> SRKKMGLLVMAYGTPYKEEDIERYYTHIRRGRKPEPEMLQDLKDRYEAIGGISPLAQITEQQAHNLEQHLNEIQDEITFKAYIGLKHIEPFIEDAVAEMHKDGITEAVSIVLAPHFSTFSVQSYNKRAKEEAEKLGGLTITSVESWYDEPKFVTYWV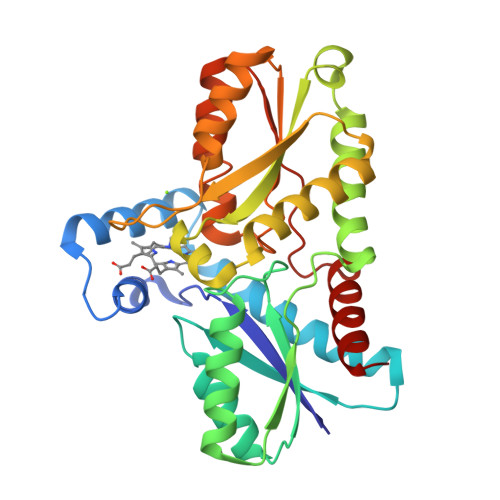DRVKETYASMPEDERENAMLIVSAASLPEKIKEFGDPYPDQLHESAKLIAEGAGVSEYAVGWQSEGNTPDPWLGPDVQDLTRDLFEQKGYQAFVYVPVGFVADHLEVLYDNDYECKVVTDDIGASYYRPEMPNAKPEFIDALATVVLKKLGR Here we describe efficient routes starting from validated parallel and antiparallel peptide assemblies to design two families of α-helical barrel proteins with central channels that bind small molecules. Computational designs are seeded by the sequences and structures of defined de novo oligomeric barrel-forming peptides, and adjacent helices are connected by loop building. For targets with antiparallel helices, short loops are sufficient. However, targets with parallel helices require longer connectors; namely, an outer layer of helix–turn–helix–turn–helix motifs that are packed onto the barrels.

We chose four protein sequences with <85% sequence identity, high pLDDT and low Rosetta energies for gene synthesis and expression in E. coli. The other protein, named sc-CC-7-LI because of its a = Leu and d = Ile core, was helical and fully resistant to heat denaturation as judged by circular dichroism spectroscopy, was monomeric according to AUC and bound dye, consistent with an accessible channel. We solved a 2.5-Å resolution X-ray structure by molecular replacement using the AlphaFold2 model for sc-CC-7-LI. For the parallel targets, the experimental structures show minor fraying at the C termini of the inner helices compared with the seeds and models, which appears to improve the packing of the external three-helix bundles. However, the symmetry of the central parallel helices is maintained. The backbone RMSD values for the repeating helix–turn–helix–turn–helix motifs are ≤0.5 Å, which is expected given the low sequence variation in the loops and the hydrophobic cores of these buttressing helices. Finally, to test the robustness of the design to mutation, we substituted all 49 a (Leu) and d (Ile) sites of the central α-helical barrel for alternative design rules for parallel heptameric α-helical barrels (that is, a = Ile and = Val). This protein (sc-CC-7-IV) was highly expressed and was also folded, as shown by circular dichroism spectroscopy and SEC-SAXS, hyperstable, monomeric and bound the reporter dye. The success rate for making single-chain constructs from these initial five parallel designs was three soluble proteins (60%) and one new α-helical barrel crystal structure (20%).

>GSHMLIAEALELIAEALFAIALALLAIAKKDKELAKKAVELAEKVYKEAEELYKKAKKKGDLIAAALALIAQALAAIALALAAIALKDKELAKKAYKLAEEVYKKAEKLYEEAKKKGDLIAAALALIAQALALIALALAAIALGDKEKLKEVIEKAKEVYKKAEELYKEAEKKGDLIAAALALIAQALALIAIALAAIALGDEETLKEVKEKAKEVYEKAKKVAEEAEKKGDLIAAALALIAQALALIAIALAAIALGDEEELKKVIEEAKKVYEEAKKIYEEAKKKGDLIAAALALIAQALALIAIALAAIALGDEETLEEARKEAEEVKKEAEELAKEAEQKGNEIAAALAEIAIALAEIAIALVEIAKK[2x]>MDFPLANLFFVPSEDATAFGRRLRAAAQQAPIVFDTAFGMPILLRKSHITTAYRDTA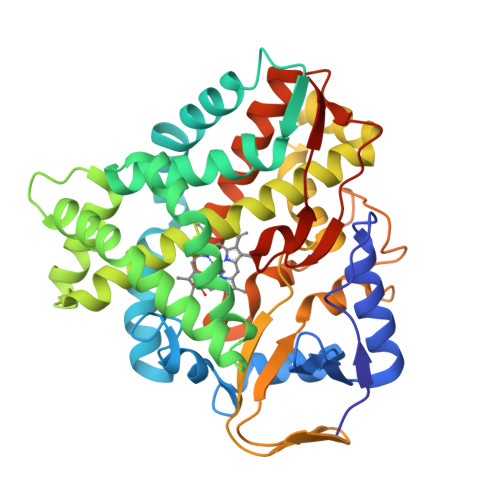TFSTRMFQAGILNGGLAAMQGDEHARMRRVYNMFFLPRAVSQYEERFVRPISEQVVDRLAGKPRVDLLEDFAMELPRRVIGELFGFPAEKLHETDERVRAMLRGLVRMHDPAAVAESQRAYGETLGLITEVVERESRDTSDTLLGEILRTLKAEHMDTIEASRQIVLSLILGGYETTSWLVANTIHALLAHPDTLARVRQDPSLLPAAIEEGMRWCPSNFGVLRMVERDVRLDDQALSAGTVVCLAGIAGNYDETAYPSPEVYDIDRKPLPAANVFGGGAHFCVGAPLARMEARVGLQALLARFPGLRAVPEERPSFMYGAKDSVAHGPDKLPVLLHHHHHHH[2x]> 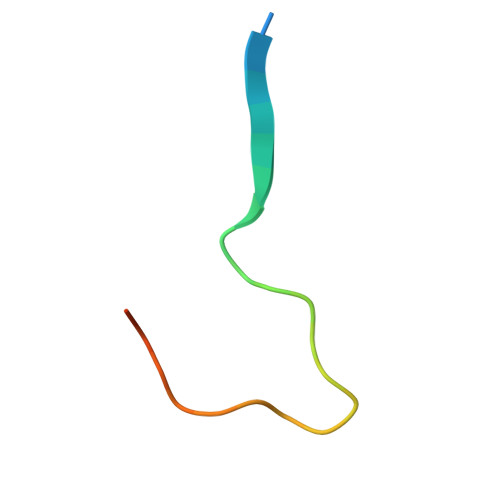MSASSGPWKPAKPAPSVSPGPWKPIPSVS>SNAQEQRMSHHYATIEVSQQLLQLLGDQLVILLRETPDGQALERSQNDFRRVLEQGRANTVDSAE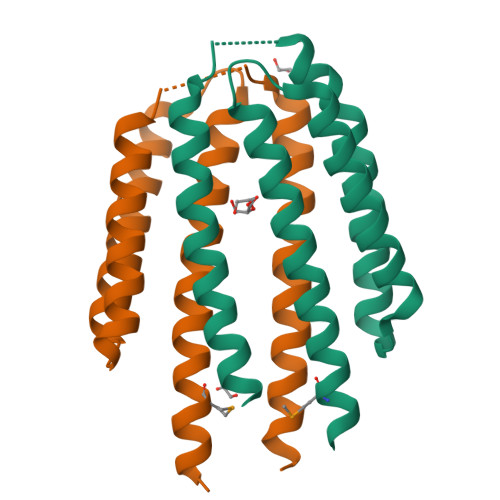QAALDGVRDAYLQLQAHTPALLEAPMADNDGFSEAFNGLRLRLQDLQQLALAGISEAETSARHRA[4x]GapR (growth-associated A/T-binding protein involved in regulation) is a chromosome structure protein conserved in α-proteobacteria, and it is discovered initially as an essential nucleoid-associated protein for normal growth and cell division in Caulobacter crescentus (1–3). Depletion of GapR gene in Caulobacter cells results in severe defects in cell growth, cell division, cell size, DNA replication, chromosome segregation/condensation and gene expression. Our current studies clearly demonstrate that free GapR is a tetramer, but not a dimer. Taken all together, there exist both major conformation and minor conformation for free GapR in solution, which are in dynamic exchange equilibrium with each other.

Interestingly, during our crystallization of GapR/10A sample, we also got a crystal which produced a dimeric structure of the Caulobacter GapR protein only, without the detection of any diffraction from DNA. A comparison of this GapR dimer structure with that of the dimer-unit from the open tetramer complex revealed that the backbone heavy atom RMSD for residues 16–65 is 0.32 Å, while residues 66–89 show larger deviations for both protomers. SAXS analysis results indicated that the experimental Rg value of the free Caulobacter GapR in solution is 28.6 Å, much larger than the calculated Rg (22.8 Å) based on this GapR dimer structure. Comparison of the calculated scattering curves from the GapR dimer structure and the experimental SAXS data of the free GapR shows a fitting χ2 value of 21.9, indicating the solution structure of free GapR can not be like this dimer structure. Analysis of the GapR dimer structure, it is apparent that the hydrophobic areas (residues 78–87) on the second α-helices are fully exposed, while the same hydrophobic areas in the closed tetramer participate in the formation of the tetrameric interface. It is possible that the dimer structure can not stably exist alone due to hydrophobic aggregation, when the C-terminal hydrophobic areas are fully exposed due to the disruption of the tetrameric interfaces for GapRΔC3, GapRD68A and GapRY82A mutants. }{}$$\begin{equation*}\ R{{\rm g}_{{\rm app}}} = \sqrt {\left( {{C_{\rm A}}Rg_{\rm A}^2 + {C_{\rm B}}Rg_{\rm B}^2} \right)/\left( {{C_{\rm A}} + {C_{\rm B}}} \right)} \end{equation*}$$\end{document} where CA and CB are the mass concentration of the major and minor conformers with radii of gyration of RgA and RgB, respectively. If the minor conformer is a dimer, then its radius gyration RgB (22.8 Å) is even smaller than RgA (26.9 Å) of the major conformer (closed tetramer), which can only result in a Rgapp that is smaller than RgA based on the above equation. Taken together, the possibility can be ruled out for the closed tetramer to dissociate into dimer in free GapR.

> MADDAIPHTDVLNSTAQGQLKSIIERVERLEVEKAEIMEQIKEVYAEAKGNGFDVKVLKKVVRIRKQDRAKRQEEDAILDLYLSAIGEILEHHHHHH> MSISISYSTTYSGWTVADYLADWSAYFGDVNHRPGQGVDGSNTGGFNPGPFDGSQYALKSTASDAAFIAGGDLHYTLFSNPSHTLWGKLDSIALGDT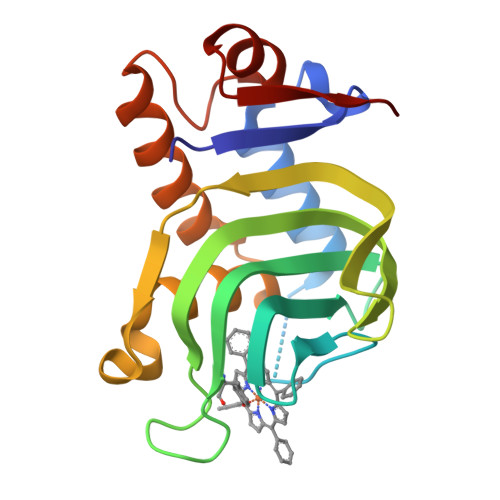LTGGASSGGYALDSQEVSFSNLGLDSPIAQGRDGTVHKVVYGLMSGDSSALQGQIDALLKAVDPSLSINSTFDQLAAAGVAHATPA Mitogen-activated protein kinase kinase kinase kinase 1 (MAP4K1) is a serine/threonine kinase that acts as an immune checkpoint downstream of T-cell receptor stimulation. MAP4K1 activity is enhanced by prostaglandin E2 (PGE2) and transforming growth factor beta (TGFβ), immune modulators commonly present in the tumor microenvironment. Therefore, its pharmacological inhibition is an attractive immuno-oncology concept for inducing therapeutic T-cell responses in cancer patients. Through its proline-rich domain, MAP4K1 binds to a diversity of adaptors in hematopoietic cells, including those involved in T-cell receptor (TCR), B-cell receptor, and cytokine-induced signaling. The function of MAP4K1 has been studied most extensively in the context of T-cell activation.

Protein X-ray crystallography confirmed that the urea moiety interacts in a bidentate hydrogen bond with the Asp101 side chain in MAP4K1 (Asp112 in the surrogate kinase MST1). Ureas synthesized from cyclic amines, which reduced overall H-bond donors by one (not shown), also displayed more than a 10-fold decrease in activity, highlighting the importance of the two hydrogen bonds for overall potency.

>[2x]GMETVQLRNPPRRQLKKLDEDSLTKQPEEVFDVLEKLGEGSYGSVYKAIHKETGQIVAIKQVPVESDLQEIIKEISIMQQCDSPHVVKYYGSYFKNTDLWIVMEYCGAGSVSDIIRLRNKTLTEDEIATILQSTLKGLEYLHFMRKIHRDIKAGNILLNTEGHAKLADFGVAGQLTDTMAKRNTVIGTPFWMAPEVIQEIGYNCVADIWSLGITAIEMAEGKPPYADIHPMRAIFMIPTNPPPTFRKPELWSDNFTDFVKQCLVKSPEQRATATQLLQHPFVRSAKGVSILRDLINEAMDVKLKRQESQQRE N-[(2S)-heptan-2-yl]formamide 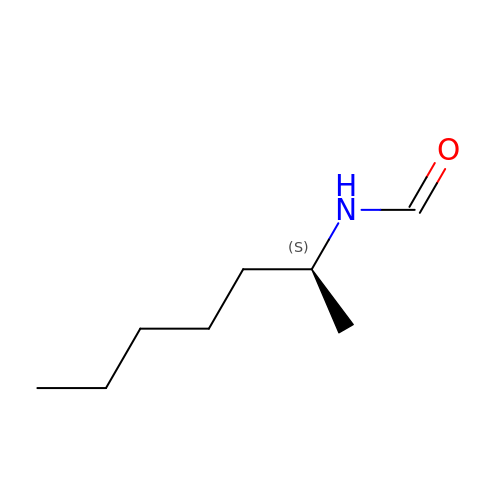| C8 H17 N O | GFVRKPKAQHTAQK-QMMMGPOBSA-N>MSKNRSSLQSGPLNSELLEEQKQEIYEAFSLFDMNNDGFLDYHELKVAMKALGFELPKREILDLIDEYDSEGRHLMKYDDFYIVMGEKILKRDPLDEIKRAFQLFDDDHTGKISIKNLRRVAKELGETLTDEELRAMIEEFDLDGDGEINENEFIAICTDS[4x];>GSKQVITEQIANDLVKEVVNSSVISIVKREFSEANYRKDFIDTMTRELYDAFLHERLYLIYMDSRAELKRNSTLKKKFFEKWQAS[4x];>[8x]MTMDTAQLKSQIQQYLVESGNYELISNELKARLLQEGWVDKVKDLTKSEMNINESTNFTQILSTVEPKALEMVSDSTRETVLKQIREFLEEIVDTQ

The yeast Sac3:Cdc31:Sus1:Thp1 (TREX-2) complex facilitates the repositioning and association of actively transcribing genes with nuclear pores (NPCs)—“gene gating”—that is central to integrating transcription, processing, and mRNA nuclear export. Sac3 is the central component of TREX-2 and contains a conserved Sac3/germinal center-associated nuclear protein (GANP) domain, which, along with the short N domain, binds both Mex67:Mtr2 and Thp1, a factor involved in transcription elongation. A region within the Sac3 C region (Sac3CID) binds Sus1 and the calmodulin-like protein, Cdc31 (Fischer et al., 2004). Sus1 is also a component of SAGA, a large complex involved in chromatin remodeling and transcription activation.

Crystals were obtained of Sac3 residues 723–805 and 753–805 complexed with both Cdc31 and Sus1. The crystals obtained with Sac3723–805 had a pseudotranslation in which one half of the asymmetric unit was shifted by close to half the unit cell, which makes structure solution more difficult because this effect greatly reduces the intensity of half of the reflections and so reduces the amount of data available. The model based on the 2.5 Å resolution P21 native data was refined to an R factor of 18.8% (Rfree 23.5%) with excellent geometry and contained Cdc31 residues 9–161, Sac3 residues 753–805 and Sus1 residues 6–95. This structure was then used to solve the Sac3723–805 crystals using molecular replacement and generated a 2.7 Å resolution model that refined to an R factor of 21.0% (Rfree 26.4%) with excellent geometry. The somewhat higher values for the R factor and Rfree for this structure were a consequence of the pseudotranslation (see Chook et al., 1998). Figures 2A and 2B and Movie S1 illustrate the structure of this complex in which Sac3 was present as a long, gently undulating α helix to which were bound one Cdc31 and two Sus1 chains. The CID region comprises Sac3 residues 723–805 and forms a gently undulating, continuous 12.5 nm α helix, which is encircled by two Sus1 chains and one Cdc31 chain. The two Sus1 binding sites on Sac3CID were designated Sus1A (residues 726–751) and Sus1B (residues 760–788). Although there were extensive interfaces between Sac3 and its three partners, there was negligible interaction between Sus1A and Sus1B or between Sus1B and Cdc31. The Sus1A chain appeared to have a slightly less intimate interaction with Sac3 than the Sus1B chain.>GPLGSMNLKAEVFLNQNCAEMMIKKAAQLILGSDLDFEYTRGVQDIQVDLGPAFMFSPDEEKTLWVSGKNQETLEKDLATLNKSSVYFFRTGTQGGAGHWQVLYYEAAKSGWVSYSSQSNHFQVTDSNGKLTASGKGLLVPHANWGKENGNYAFLLVNASAENIIHAANFVYILRTQNEVAAIEYCALNHEFHPEIKR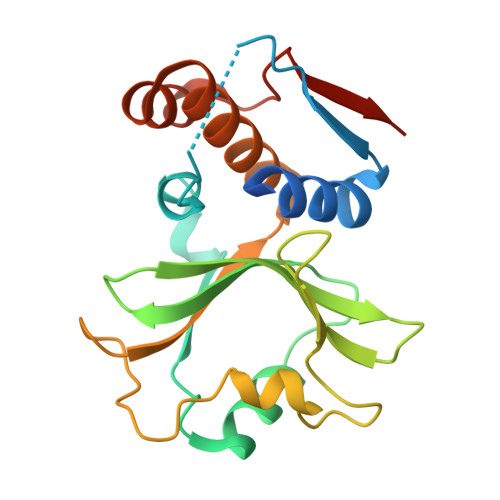TARAKAE[2x]2-(3-oxidanyl-2-oxidanylidene-pyridin-1-yl)-~{N}-[2-(4-phenylphenyl)ethyl]ethanamide | 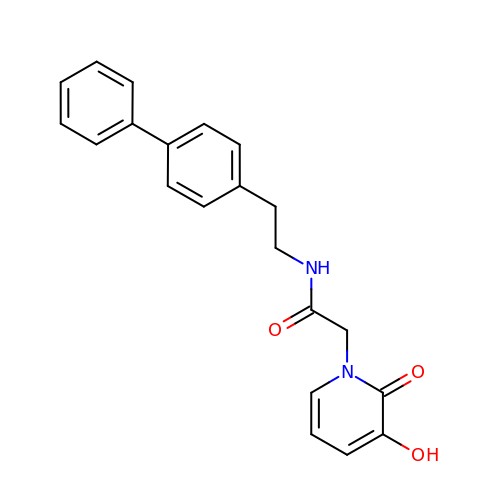C21 H20 N2 O3 | XKRQSRFKBWMVSU-UHFFFAOYSA-N>MSIFPTRDSRDLSSRRRSLIDWEFPQMALVPLDQVFDWAERSRQSLHDDIVNMHRNLFSLEPFTAMDNAFESVMKEMSAIQPREFHPELEYTQPGELDFLKDAYEVGKDGRLHFKVYFNVKNFKAEEITIKADKNKLVVRAQKSVACGDAAMSESVGRSIPLPPSVDRNHIQATITTDDVLVIEAPVNEPNYKAIKLSPEKGLAIQPSEVQERQLAVKNKEGLEIVTAEDGSKKIHLELKVDPHFAPKDVKVWAKGNKVYVHGVTGKEEKTENASHSEHREFYKAFVT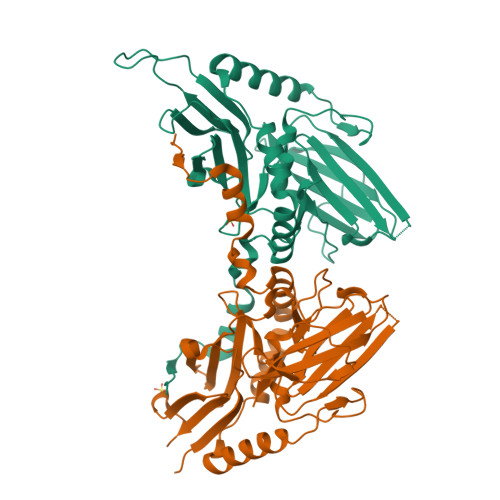PEVVDASKTQAEIVDGLMVVEAPLFK[2x]> GMSWQAYVDDHLLCDIEGQHLSAAAIVGHDGSVWAQSENFPELKPEEVAGMIKDFDEPGTLAPTGLFVGGTKYMVI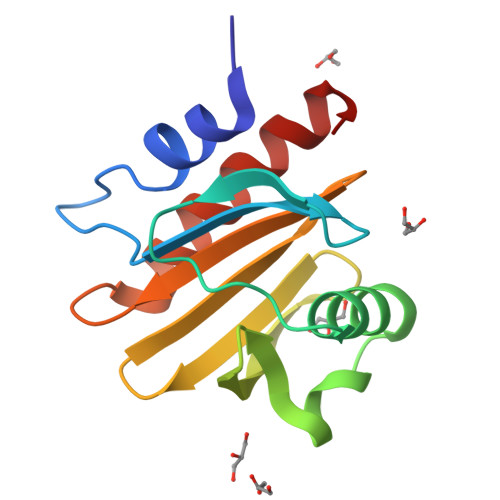QGEPGVVIRGKKGTGGITIKKTGMSLIIGIYDEPMTPGQCNMVVERLGDYLIEQGF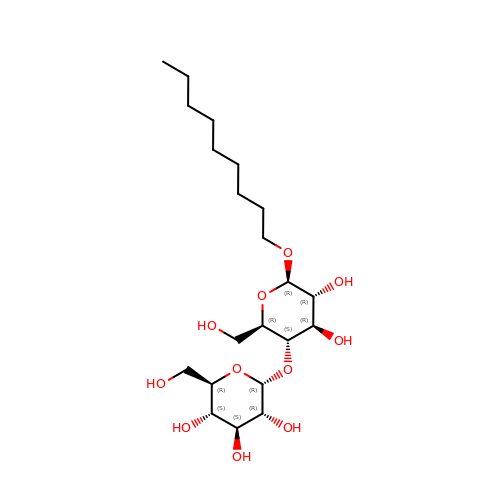nonyl 4-O-alpha-D-glucopyranosyl-beta-D-glucopyranoside | C21 H40 O11 | KCCBGPCYGBPHBR-ZESVGKPKSA-N4-HYDROXY-LYSINE | C6 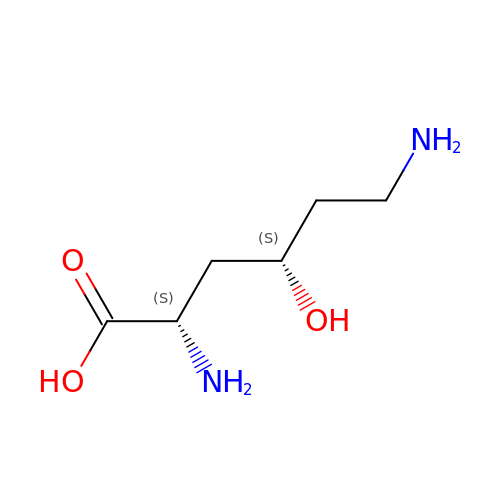H14 N2 O3 | ASYBZHICIMVQII-WHFBIAKZSA-N>[2x]ALSAEGSSGGSRGGSPKAEAASVPSWPQILGRLTDNRDLARGQAAWAMDQIMTGNARPAQIA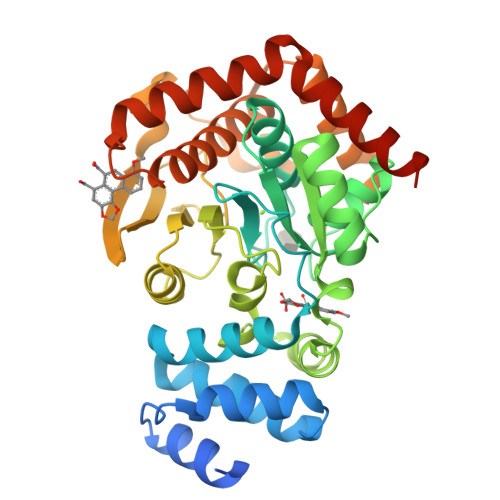AFAVAMTMKAPTADEVGELAGVMLSHAHPLPADTVPDDAVDVVGTGGDGVNTVNLSTMAAIVVAAAGVPVVKHGNRAASSLSGGADTLEALGVRIDLGPDLVARSLAEVGIGFCFAPRFHPSYRHAAAVRREIGVPTVFNLLGPLTNPARPRAGLIGCAFADLAEVMAGVFAARRSSVLVVHGDDGLDELTTTTTSTIWRVAAGSVDKLTFDPAGFGFARAQLDQLAGGDAQANAAAVRAVLGGARGPVRDAVVLNAAGAIVAHAGLSSRAEWLPAWEEGLRRASAAIDTGAAEQLLARWVRFGRQILEHHHHHH> NPIHDRTSDYHKYLKVKQGDSDLFKLTVSDKRYIWYNPDPKERDSYECGEIVSETSDSFTFKTVDGQDRQVKKDDANQRNPIKFDGVEDMSELSYLNEPAVFHNLRVRYNQDLIYTYSGLFLVAVNPFKRIPIYTQEMVDIFKGRRRNEVAPHIFAISDVAYRSMLDDRQNQSLLITGESGAGKTENTKKVIQYLASVAGRNQANGSGVLEQQILQANPILEAFGNAKTTRNNNSSRFGKFIEIQFNSAGFISGASIQSYLLEKSRVVFQSETERNYHIFYQLLAGATAEEKKALHLAGPESFNYLNQSGCVDIKGVSDSEEFKITRQAMDIVGFSQEEQMSIFKIIAGILHLGNIKFEKGAGEGAVLKDKTALNAASTVFGVNPSVLEKALMEPRILAGRDLVAQHLNVEKSSSSRDALVKALYGRLFLWLVKKINNVLCQERKAYFIGVLDISGFEIFKVNSFEQLCINYTNEKLQQFFNHHMFKLEQEEYLKEKINWTFIDFGLDSQATIDLIDGRQPPGILALLDEQSVFPNATDNTLITKLH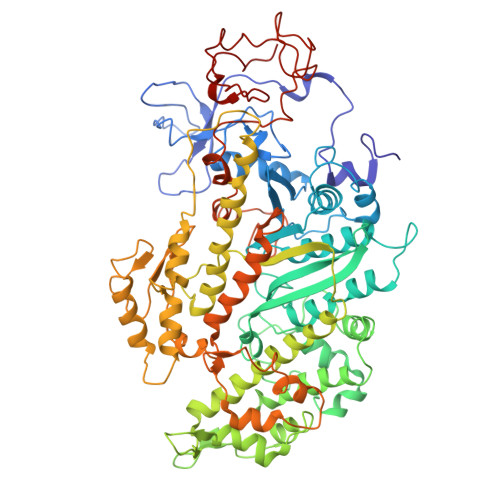SHFSKKNAKYEEPRFSKTEFGVTHYAGQVMYEIQDWLEKNKDPLQQDLELCFKDSSDNVVTKLFNDPNIASRAKKGANFITVAAQYKEQLASLMATLETTNPHFVRCIIPNNKQLPAKLEDKVVLDQLRCNVVLEGIRITRKGFPNRIIYADFVKRYYLLAPNVPRDAEDSQKATDAVLKHLNIDPEQYRFGITKIFFRAGQLARIEEARE> MAHHHHHMVINLAYDDNGTGDPVVFIAGRGGAGRTWHPHQVPAFLAAGYRCITFDNRGIGATENAEGFTTQTMVADTAALIETLDIAPARVVGVSMGAFIAQELMVVAPELVSSAVLMATRGRLDRARQFFNKAEAELYDSGVQLPPTYDARARLLENFSRKTLNDDVAVGDWIAMFSM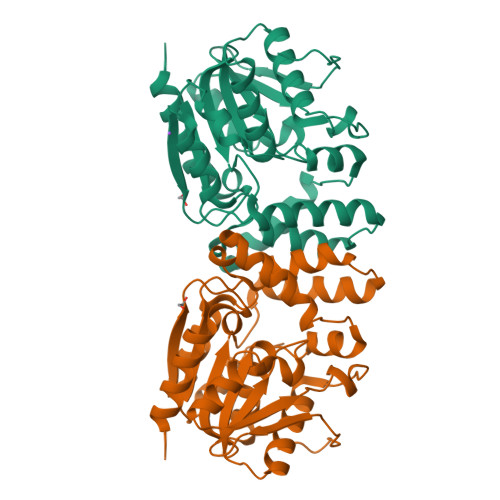WPIKSTPGLRCQLDCAPQTYRLPAYRNIAAPVLVIGFADDVVTPPYLGREVADALPNGRYLQIPDAGHLGFFERPEAVNTAMLKFFASVKA> NTVTEDTPATEQAVETPQPTAVSEEAPSSSKETKIPQTPGDAEETVADDANDLAPQAPAKTADTPATSKATIRDLNDPSQVKTLQEKAGKGAGTVVAVIDAGFDKNHEAWRLTDKTKARYQSKEDLEKAKKEHGITYGEWVNDKVAYYHDYSKDGKTAVDQEHGTHVSGILSGNAPSETKEPYRLEGAMPEAQLLLMRVEIVNGLADYARNYAQAIRDAVNLGAKVINMSFGNAALAYANLPDETKKAFDYAKSKGVSIVTSAGNDSSFGGKTRLPLADHPDYGVVGTPAAADSTLTVASYSPDKQLTETATVKTDDHQAKEMPVLSTNRFEPNKAYDYAYANRGMKEDDFKDVKGKIALIERGDIDFKDKIANAKKAGAVGVLIYDNQDKGFPIELPNVDQMPAAFISRKDGLLLKDNSKKTITFNATPKVLPTASDTKLSRFSSWGLTADGNIKPDIAAPGQDILSSVANNKYAKLSGTAMSAPLVAGIMGLLQKQYETQYPDMTPSERLDLAKKVLMSSATALYDEDEKAYFSPRQQGAGAVDAKKASAATMYVTDKDNTSSKVHLNNVSDKFEVTVTVHNKSDKPQELYYQATVQTDKVDGKHFALAPKALYETSWQKITIPANSSKQVTVPIDASRFSKDLLAQMKNGYFLEGFVRFKQDPKKEELMSIPYIGFRGDFGNLSALEKPIYDSKDGSSYYHEANSDAKDQLDGDGLQFYALKNNFTALTTESNPWTIIKAVKEGVENIEDIESSEITETIFAGTFAKQDDDSHYYIHRHANGKPYAAISPNGDGNRDYVQFQGTFLRNAKNLVAEVLDKEGNVVWTSEVTEQVVKNYNNDLASTLGSTRFEKTRWDGKDKDGKVVVNGTYTYRVRYTPISSGAKEQHTDFDVIVDNTTPEVATSATFSTEDRRLTLASKPKTSQPIYRERIAYTYMDEDLPTTEYISPNEDGTFTLPEEAETMEGGTVPLKMSDFTYVVEDMAGNITYTPVTKLLEGHS

The ScpA enzyme is one of two multi-domain cell envelope proteases (CEPs) produced by the Gram-positive bacterium Streptococcus pyogenes. ScpA inactivation of human C5a (hC5a) results from a single proteolytic event between residues H67 and K68, releasing the 7 C-terminal (C-ter) residues of the chemotaxin associated with receptor activation. The structure of ScpA showed that it is a subtilisin-like protease with a PA domain inserted within the catalytic domain and 3 tandemly arranged C-terminal fibronectin type III domains (Fn1-Fn3). Based on proximity to the active site, the PA and Fn2 domains were proposed to participate in substrate interactions in the active site and at an exosite respectively.

To circumvent potential complexities expected when measuring substrate binding to an active enzyme, surface plasmon resonance (SPR) studies utilized the S512A active site mutant of ScpA (ScpAS512A) and recombinant His-tagged C5a peptides. The sensorgrams observed for ScpAS512A binding to immobilized rhC5a were well accounted for with global fitting of the data using a 1:1 Langmuir binding model. The equilibrium dissociation constant (KD) derived from these kinetic parameters was in the low nM range (34 nM) indicating that ScpA has a high affinity for rhC5a. The analysis confirms that the substrate binds to ScpA at a single site with high affinity (KDITC = 30.8 nM). The ITC measurements also indicated that the binding of the substrate is an enthalpically driven process with a ΔH of −9.4 kcal/mol and ΔS of 2.3 cal/mol/deg. Binding of ScpA to the larger core portion of C5a (rhC5acore) was also measured by SPR. rhC5acore represents the larger N-terminal product (PN) of ScpA inactivation. Thus, the high affinity binding of rhC5acore along with the competitive binding data indicated that the bulk of substrate interactions occur at a site outside of the ScpA active site (i.e. an exosite). ScpAS512A binds to rhC5adR with a KD of 191 nM, intermediate in value between the KDs for rhC5a and rhC5acore.>[4x]MADQAMTDQDQGAVTLYSGTAITDAKKNHPFSVKVGLAQVLRGGAIVEVSSVNQAKLAESAGACSVIVSDPVRSRGGVRRMPDPVLIKEVKRAVSVPVMARARVGHFVEAQILESLAVDYIDESEIISVADDDHFINKHNFRSPFICGCRDTGEALRRIREGAAMIRIQGDLTATGNIAETVKNVRSLMGEVRVLNNMDDDEVFTFAKKISAPYDLVAQTKQMGRVPVVQFASGGITTPADAALMMQLGCDGVFVGSEVFDGPDPFKKLRSIVQAVQHYNDPHVLAEMSSGLENAMESLNVRGDRIQDFGQGSVHHHHHH;>SPFSVKVGLAQMLRGGVIMDVVNAEQARIAEEAGACAVMALERVPADIRAQGGVARMSDPQMIKEIKQAVTIPVMAKARIGHFVEAQILEAIGIDYIDESEVLTLADEDHHINKHNFRIPFVCGCRNLGEAL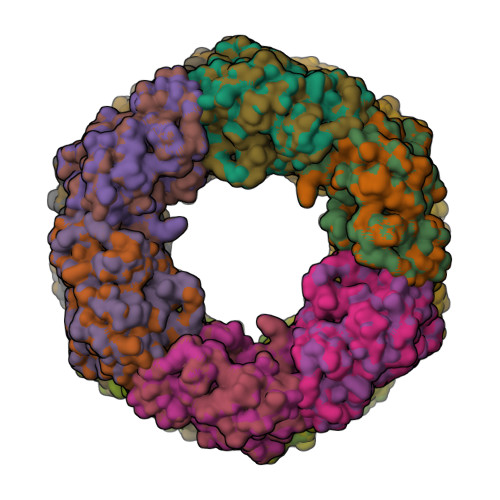RRIREGAAMIRTKGEAGTGNIIEAVRHVRSVNGDIRVLRNMDDDEVFTFAKKLAAPYDLVMQTKQLGRLPVVQFAAGGVATPADAALMMQLGCDGVFVGSGIFKSGDPARRARAIVQAVTHYSDPEMLVEVSCGLGEAM[4x]The first procapsid form, prohead I, is built from 775 copies of the head protein pb8 arranged into 11 pentamers and 120 hexamers, as well as a dodecamer of the portal protein pb7 located at the 12th vertex. The DNA-filled capsid is decorated with 120 copies of the 17.3 kDa protein pb10, which binds as a monomer to the centre of each hexamer. Basic principles of T5 capsid assembly and maturation have been established and follow the phage HK97 paradigm. Here we investigate the properties of pb10, the decoration protein of bacteriophage T5 capsid.

To explore the nature of the interaction between pb10 and the major capsid protein pb8, we first searched for the position of pb10 on capsid structures determined by cryo-electron microscopy and image reconstruction. Two density regions corresponding to a single hexamer of the empty expanded capsid observed without and with pb10 were obtained (estimated resolution of 8 and 9 Å, respectively). Pb8 adopts the major capsid protein fold first observed in the X-ray structure of the phage HK97 capsid, and its 3D structure was modelled on this basis. Six copies of this pb8 model were fit into the density of one hexamer in both cryoEM maps and the density corresponding to pb10 was identified. We did not observe any additional density inside the capsid in the map of the pb10-bound capsid, showing that pb10 is located at the outer surface of the capsid. The density corresponding to pb10 observed at the centre of each pb8 hexamer has a size compatible with the NTD of pb10. It appears as an averaged low-resolution lump, likely due to the superposition of one pb10 monomer in each of 6 quasi-equivalent positions on the hexamer. The CTD density is not distinguishable from the noise, suggesting that its position relative to the capsid is variable. The centre of the hexamers is formed by six copies of the A-loop of pb8 (named by homology with the equivalent loop in the HK97 capsid protein) and its surface is negatively charged due to the presence of multiple aspartate and glutamate residues in these loops. No shift of the non-expanded procapsid band was observed in the presence of pb10. This shows that the structural reorganization of the capsid protein subunits that takes place upon expansion creates the binding sites for the decoration protein, as observed in other phages.

>AVNQSSSVEVSSESYETIFSQRIIRDLQKELVVGALFEELPMSSKILTMLVEPDAGKATWVAASTYGTDTTTGEEVKGALKEIHFSTYKLAAKSFITDETEEDAIFSLLPLLRKRLIEAHAVSIEEAFMTGDGSGKPKGLLTLASEDSAKVVTEAKADGSVLVTAKTISKLRRKLGRHGLKLSKLVLIVSMDAYYDLLEDEEWQDVAQVGNDSVKLQGQVGRIYGLPVVVSEYFPAKANSAEFAVIVYKDNFVMPRQRAVTVERERQAGKQRDAYYVTQRVNLQRYFANGVVSGTYAAS[6x]>HHHHHHMKKVNNDTVFGILQL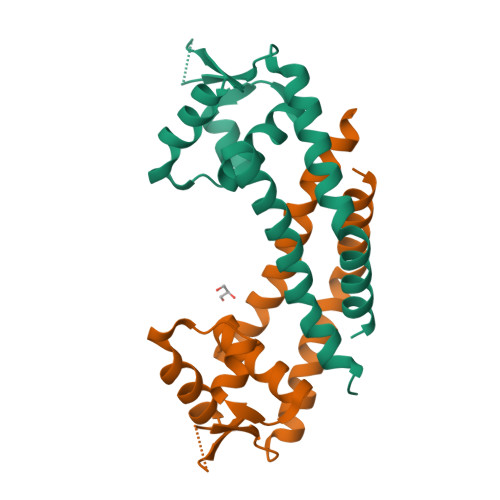ETLLGDINSIFSEIESEYKMSREEILILLTLWQKGSMTLKEMDRFVEVKPYKRTRTYNNLVELEWIYKERPVDDERTVIIHFNEKLQQEKVELLNFISDAIASRATAMQNSLNAIIAV[2x]> GAGEARLEEAVNRWVLKFYFHEALRAFRGSRYGDFRQIRDIMQALLVRPLGKEHTVSRLLRVMQCLSRIEEGENLDCSFDMEAELTPLESAINVLEMIKTEFTLTE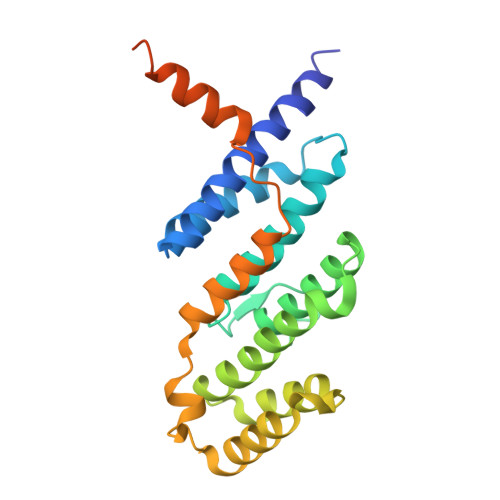AVVESSRKLVKEAAVIICIKNKEFEKASKILKKHMSKDPTTQKLRNDLLNIIREKNLAHPVIQNFSYETFQQKMLRFLESHLDDAEPYLLTMAKKALKSESAASSTGKEDKQPAPGPVEKPPREPARQL>[4x]MIKVTVTNSFFE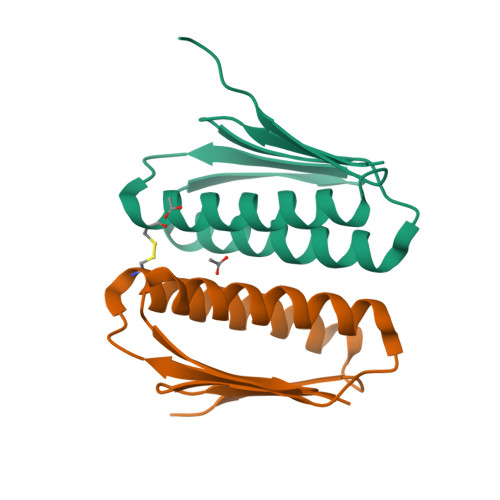VTGHAPDKTLCASVSLLTQHVANFLKAEKKAKIKKESGYLKVKFEELENCEVKVLAAMVRSLKELEQKFPSQIRVEVIDNGS The circadian clock of the cyanobacterium Synechococcus elongatus can be reconstituted in vitro by three proteins, KaiA, KaiB and KaiC. Homo-hexameric KaiC displays kinase, phosphatase and ATPase activities; KaiA enhances KaiC phosphorylation and KaiB antagonizes KaiA. The crystal structure of KaiC from S. elongatus revealed a hexamer in the shape of a double doughnut with approximate dimensions 100×100 Å, whereby the N-terminal CI and C-terminal CII halves of subunits are joined by a 15-amino acid linker. Two phosphorylation sites (P-sites), T432 and S431 that are both located in the CII half were identified in KaiC.

To analyze the phosphorylation patterns of KaiC P-site mutants and to visualize potential conformational variations in the vicinity of bound ATP and residues 432 and 431 at hexamer subunit interfaces, we determined crystal structures of the S. elongatus KaiC single mutants T432A (TSa), S431A (TaT), S431D (TdT), and T426N (nST) and the double mutants T426A/T432A (aSa) and S431A/T432E (Tae). b KaiC mutations xyz or mutants KaiCxyz are sequentially shown in order of sites x = 426, y = 431, and z = 432 where the wild-type residue is in upper case and mutated residues are shown in lower case, i.e. Tsa or KaiCTSa, where the residue at position 426 is T, the residue at position 431 is S, and the residue at position 432 is mutated to A. The crystal structures of the KaiCTaT and KaiCTae mutants are noteworthy in two respects. The structures of the Tae and TaT mutants reveal that T426 residues in some of the six subunits carry a phosphate group and call into question the common assumption of just two P-sites in the core clock protein. Among the structures of the six KaiC mutant proteins reported here, those of the TaT and Tae mutants are the most intriguing because they imply that T426 can be a third phosphorylation site. The observation of a phosphate at T426 in the crystals but not under other conditions, i.e. SDS-PAGE assays using heated KaiCTae samples or mass spectrometric analyses of wt-KaiC may indicate that phosphorylation at this site is labile. However, we believe that the conditions for growing KaiC crystals promote increased phosphorylation levels relative to protein isolated from in vitro cycling reactions or incubated with ATP at elevated temperatures. The kinase activity of KaiC is enhanced under acidic conditions, resulting in transfer of ATPγS thiophosphate groups to T432, S431 or T426. Therefore, phosphorylation at T426 seen in selected subunits of the Tae and TaT mutants is most likely not a crystallographic artifact. Rather the crystal structures have preserved a third P-site in KaiCII that appears to have evaded identification by other approaches.

>[6x]MTSAEMTSPNNNSEHQAIAKMRTMIEGFDDISHGGLPIGRSTLVSGTSGTGKTLFSIQFLYNGIIEFDEPGVFVTFEETPQDIIKNARSFGWDLAKLVDEGKLFILDASPDPEGQEVVGGFDLSALIERINYAIQKYRARRVSIDSVTSVFQQYDASSVVRRELFRLVARLKQIGATTVMTTERIEEYGPIARYGVEEFVSDNVVILRNVLEGERRRRTLEILKLRGTSHMKGEYPFTITDHGINIFPLGAMRLTQRSSNVRVSSGVVRLDEMCGGGFFKDSIILATGATGTGKTLLVSRFVENACANKERAILFAYEESRAQLLRNAYSWGMDFEEMERQNLLKIVCAYPESAGLEDHLQIIKSEINDFKPARIAIDSLSALARGVSNNAFRQFVIGVTGYAKQEEITGLFTNTSDQFMGAHSITDSHIAEITDTIILLQYVEIRGEMSRAINVFKMRGSWHDKAIREFMISDKGPDIKDSFRNFERIISGSPTRITVDEKSELSRIVRGVQEKGPES>MGAMIVKEVYETAEKIKSMEIRGAGRIARAAAQALMIQAEKSKAKEPEELWNELKVASKILYNTRPTAVSLPNALRYVMHRVKAAYLGGADLETLRFTAINSAKEFIYNSEKAIERIGEIGAKRIEDGDIIMTHCHSKAAISVMKKAFEQGKNIKVIVTETRPKWQGKITAKELASYGIPVIYIVDSAARHYMKMTDKVVMGANSITANGAVINKIGTSLIALTAKEHRVWVMIAAETYKFHPATMLGQLVEIEMRDPTEVIPEEELRTWPKNIEVWNPAFDVTPPEYIDVIITERGIIPPYAAIDILKEEFGWALKYKEPWED[3x]

In summary, our study demonstrates that PH0208 protein would function as a purine nucleotide dependent R15Pi enzyme and not as a homologue of the regulatory subunit of eIF2B. In NMP degradation pathway, R15Pi catalyzes the conversion of ribose-1,5-bisphosphate (R15P, substrate) into ribulose-1,5-bisphosphate (RuBP, product) in an adenosine 5′-monophosphate (AMP)-dependent manner. AMP acts as an activator of R15Pi and in its absence the enzymatic activity has been found to decline dramatically. Monomer of PH0208 protein consists of an N-terminal α-helical domain (residues 1–122) and a C-terminal α-β-α sandwich domain (residues 123–324).

To verify the preferred molecule at the ‘AMP binding site’, PH0208-WT, PH0208-C135S and PH0208-D204N were crystallized in the presence of both AMP and GMP. In the presence of both the potential ligands, AMP outcompete GMP and binds to the ‘AMP binding site’ utilizing the similar set of amino acid while GMP binds to the ‘GMP binding loop’. During crystallization, even a higher concentration of GMP (4.5 mM) as compared to AMP (1.5 mM) could not aid GMP to occupy the ‘AMP binding site’. This further indicates a higher affinity of AMP at the ‘AMP binding site’. Evidently, when both AMP and GMP were made available, AMP binds to the ‘AMP binding site’ with a higher preference than GMP, while GMP occupies the ‘GMP binding loop’ only. Binding of GMP to the ‘GMP binding loop’ involves very few interactions which predominantly includes only the guanosine base ring of the GMP molecule. Thus, it might also be possible that the binding of GMP to the ‘GMP binding loop’ is an outcome of crystallization artifact. Both, AMP and GMP bind to PH0208 protein even after the mutation of the catalytic residues (PH0208-C135S and PH0208-D204N) at the active site pocket.> MKFGNFLLTYQPPELSQTEVMKRLVNLGKASEGCGFDTVWLLEHHFTEFGLLGNPYVAAAHLLGATETLNVGTAAIVLPTAHPVRQAEDVNLLDQMSKGRFRFGICRGLYDKDFRVFGTDMDNSRALMDCWYDLMKEGFNEGYIAADNEHIKFPKIQLNPSAYTQGGAPVYVVAESASTTEWAAERGLPMILSWIINTHEKKAQLDLYNEVATEHGYDVTKIDHCLSYITSVDHDSNRAKDICRNFLGHWYDSYVNATKIFDDSDQTKGYDFNKGQWRDFVLKGHKDTNRRIDYSYEINPVGTPEECIAIIQQDIDATGIDNICCGFEANGSEEEI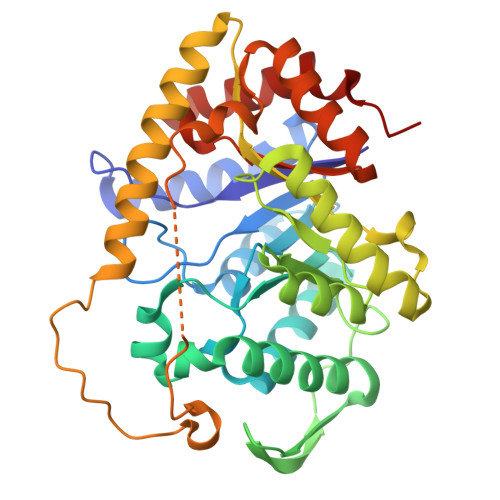IASMKLFQSDVMPYLKEKQ> 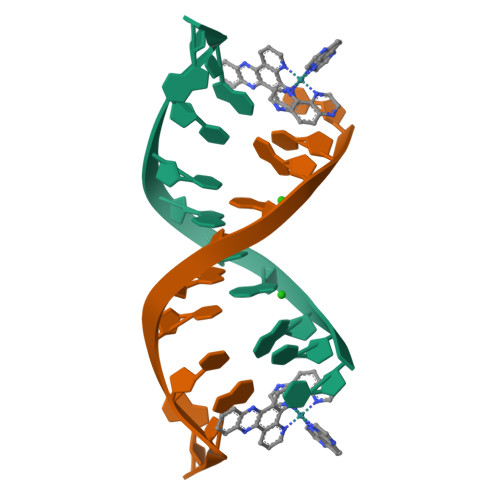XTGGCGCCAA>VKQVFNFNAGPSALPKPALERAQKELLNFNDTQMSVMELSHRSQSYEEVHEQAQNLLRELLQIPNDYQILFLQGGASLQFTMLPMNLLTKGTIGNYVLTGSWSEKALKEAKLLGETHIAASTKANSYQSIPDFSEFQLNENDAYLHITSNNTIYGTQYQNFPEINHAPLIADMSSDILSRPLKVNQFGMIYAGAQKNLGPSGVTVVIVKKDLLNTKVEQVPTMLQYATHIKSDSLYNTPPTFSIYMLRNVLDWIKDLGGAEAIAKQNEEKAKIIYDTIDESNGFYVGHAEKGSRSLMNVTFNLR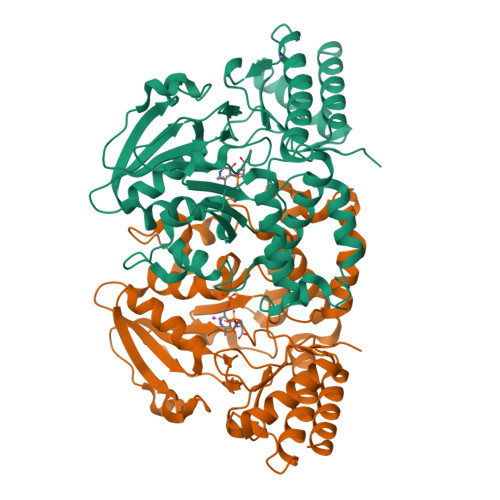NEELNQQFLAKAKEQGFVGLNGHRSVGGCRASIYNAVPIDACIALRELMIQFKENA[2x]2-[(1-methyl-2-oxidanyl-4-oxidanylidene-quinolin-3-yl)carbonylamino]ethanoic acid | C13 H12 N2 O5 | 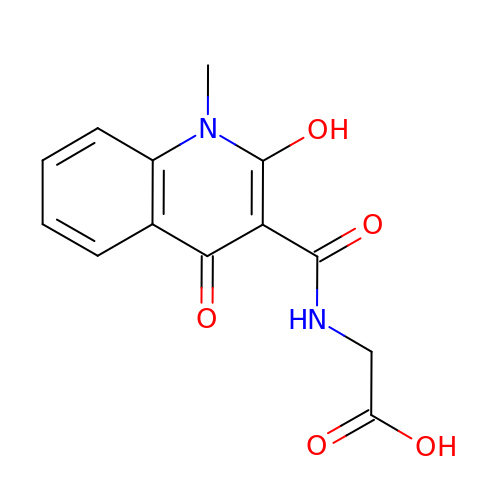CRTHWBYRFGFTNO-UHFFFAOYSA-N> 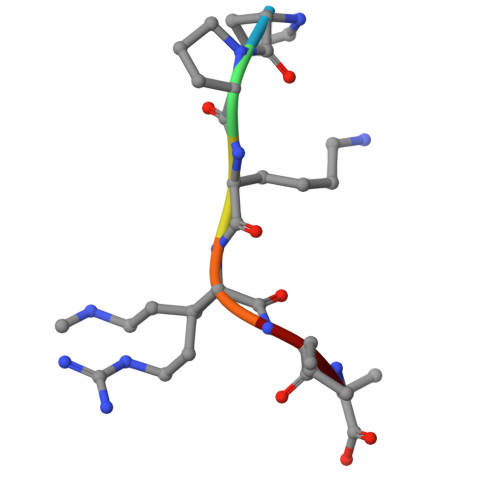PPKRIA>[2x]MTWRRFDVAYHDPDLDRLILAARPLLSESPGR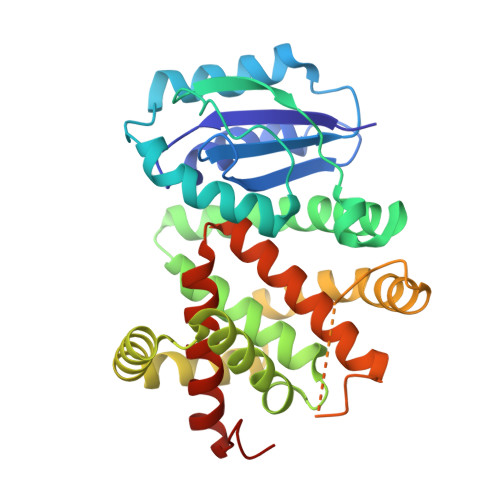SWFQRHWVRGPHLELWFDHPEPSWERVREVLGTHLRAHPSRTRIDPDRLLPQHRRLALAEQIDEPLLPFYDDNTLHRAVPRSRVHVLGSAAAEDLFHDFHAAASTAAFDQLDAVVAGESRLGLAFELMIAAAHAHAEGGITGGFVSFRSHAEAFLAGAAGLRERWEAEYRTRAEALRAQVAAVVTGTPRGRAWTGLLDGFAGRGDELIASGALTVEPASPTAAAEPDTEFHRALRANRTWHDEVLRSPSFRRYRLLLNLTFLQMSRLGVTAVQRSLLCHFAASAVEEEYGVSAIEIAVGGM In archaea, early branching bacteria, and amitochondrial eukaryotes, the reactions are catalyzed by a much simpler enzyme, 2-oxoacid:ferredoxin oxidoreductase (OFOR). In this study, we report the crystal structures of StOFOR1 and its paralog StOFOR2 (STK_24350 and STK_24330), providing insights into the substrate recognition and reaction mechanism of the (ab)2 type OFORs from extremophilic archaea and bacteria. StOFOR2 and StOFOR1 possess domains III (1a–228a), I (228a–500a), and II (500a–627/628a) of the a-subunit and domain VI (1b–305b) of b-subunit but lack domains IV, V, and VII. The TPP molecules of StOFORs accompany a Mg2+ ion around their pyrophosphate group and are buried at the interface between the a-subunits and b-subunits.

STK_24350 (a-subunit) and STK_24330 (b-subunit) have similar domain architectures to STK_23000 and STK_22980, with high amino acid sequence identity for both subunits (59% and 71%). The recombinant protein showed broad OFOR activities toward pyruvate and 2-oxoglutarate; therefore, we designated this enzyme as StOFOR2. However, StOFOR2 has less activity compared with StOFOR1, due to its relatively higher Km towards both substrates. In contrast, StOFOR2 easily formed high-quality single crystals in solutions containing ammonium salts as the precipitant. We could solve the structure of StOFOR2 by the single-wavelength anomalous dispersion method using a selenomethionine(SeMet)-labeled protein crystal, and we determined the structures of the ligand-free (2.1 Å resolution) and pyruvate-complexed (2.2 Å) forms. A database search using Dali server indicated that StOFOR2 is structurally similar to MtOOR (Z-score = 39.1, RMSD = 2.6 Å, and Nalign = 346 for a-subunit, and Z-score = 21.4, RMSD = 2.3 Å, and Nalign = 206 for b-subunit) and DaPFOR (Z-score = 37.6, RMSD = 2.7 Å, and Nalign = 346 for a-subunit, and Z-score = 19.6, RMSD = 2.6 Å, and Nalign = 222 for b-subunit). We used the StOFOR2 structure to investigate its possible interactions with StFd because it has better quality than StOFOR1 at the molecular surface. StFd was modeled into the large pocket of StOFOR2 by aligning the two iron-sulfur clusters onto those of the Fd-like domain V of DaPFOR. Cluster I is located 14 Å from the sole [4Fe-4S] cluster in StOFOR2, and the gap is filled with loops near the clusters. Loops between cluster I in StFd and the sole cluster in StOFOR2 simultaneously provide a protein-protein interface and an electron transfer pathway. The loops from the two proteins mainly interact via hydrophobic residues, involving the side chains of Ile46 and Pro94 from StFd and Pro13b and Phe18b from StOFOR2.

> MTRIVWMIGGAQGLGVDTSANIFGNAVAKAGYYLFGNREYYSNIKGRHSYFEVVISEKPIRSLSSYVNILASFDAETVFQHFTETKEYLIYNVEYENTTVDLVKSMEPEMAEQVKEALSKERLGFTIKDVLEYLKRRGVKVIGFNYTELIKKIADTFKVPMSVVERAKNMIAVGASYGLLGLKFDYLKDAISSTFKNELFIKFNTMAAELGYNSVPNVYKLQEYKIEKQRIQVDGNTISAMGKLAGGLRFQSYYPITPASDESVYIEANQNLDMIVEGNELRKGGVVVVQAEDELAAINMAVGAALTGVRSATATSGPGFSLMSEGISWAGMNEVPVVITYYMRGAPATGLPTRSGQADLKFALNVGHGEFPRIVIASGDHVEIFWDAIWALNLAEKYQTPVIHIIEKTLANAYSVFEEELITNRPYVIERGKIVKPTSDYFNRFEVTEDGISPRVFLGQASIFYTGDEHNEEGHITENSINRMKMYEKRNKKLETADKEIPEEQRVNIVGDADIVLLTWGSPKGAILDAMEELSKDGIKTMMVQVKMFNPYPKNLMKKILSGKSKIIAVENNYNAQGAEVLAEKTGIFATNYILKWTGRPITREEVIEGIKKILERDEKRVVLYGGA;> MVERKPVFVDWCPGCGDFGILRAEEMAIRELGINPKSVVIVSGIGCSGKIPHFMNLPISGVHTLHGRSIAFATGIKLSNPSLEVIVNVGDGDGLGIGMGHFVHLGRRNIDIAVLVHNNGVYGLTKGQASPTLHRGEKTKSLPKPNIMDAVNPLAVALAAGYTFVARGYAYDVMHLKELIKKAILHKGSALVDILQPCPTYNDINTKEWYDKRVYKLDNVPGWDPVVRKEEEAQKKFEQAIMKSYEWGEKIPIGIFYQNELVPTFEDRLTSNIPNYREYYPAKQQIEINGISTTKIDELIKAKRI>GAASKKVNVLVVGLDNSGKTTIIERLKPRPRQAAEVAPTVGFTVDEVEKGPLTFTVFDMSGAGRYRTLWEQYYREADAVVFVVDSADKLRMVVARDEMEHMLKHSNMRKVPILYFANKKDLPVAMP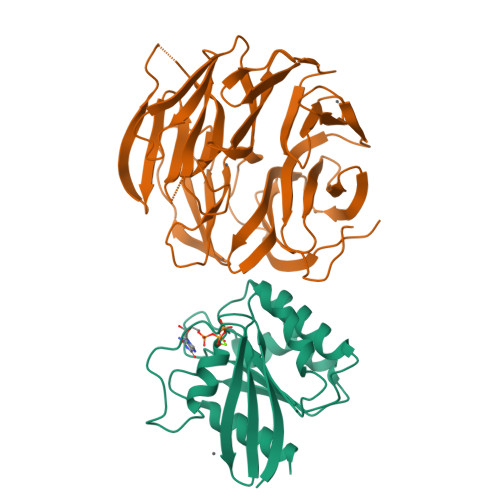PVEIAQALGLDDIKDRPWQIVPSNGLTGEGVDKGIDWLAERLS[4x];>[4x]MVHESNPNDYAAGDAGNASGRYTTGSNGIPPMLPSVRSVWLDAFNDPVAGISAYTPCVHTCNLFGDGENRLVIADEDRKLKIWKGTQKASEHPLLDTPVAICSYISENTAPRLPALAVAAGSHIYIYRNLRPYYKFVLPPENVNTEEQDIWQKVMEGEIVIGEAVAQLTRLQVRAGDAGVVLQTRSLQLMNIGDPDAKMAFVEHWQGQPLVATTVITCMDVVKQAIDEPDAVSCLVVGTESGRILILNPAGTAIVKNIWVGITPAMIAVQGELDVGYRITVAGRDGKLYHIRNGELSQTIIQLEAQPVGLVRLAKHVAVGCMNDVVHAYTPTGHKSWSLYLPCHILAMQRMEVTGQRNTKALIVALSNGEVRVYNEKLLVSVHVSPNPVTALWFGRYGREDNTLLAITKSGALDIKMLPRTANLE> MGKKNSKLKQD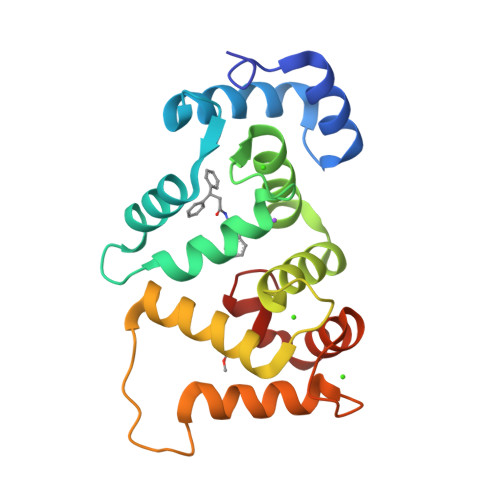TIDRLTTDTYFTEKEIRQWHKGFLKDCPNGLLTEQGFIKIYKQFFPDGDPSKFASLVFRVFDENNDGAIEFEEFIRALSITSRGNLDEKLHWAFRLYDVDNDGYITREEMYNIVDAIYQMVGQQPQTEDENTPQKRVDKIFDQMDKNHDDRLTLEEFREGSKADPRMVQALSLGGD> DRVTTQTAGNTAINTQSSLGVLCAYVEDPTKSDPPSSSTDQPTTTFTAIDRWYTGRLNSWTKAVKTFSFQAVPLPGAFLSRQGGLNGGAFTATLHRHFLMKCGWQVQVQCNLTQFHQGALLVAMVPETTLDVKPDGKAKSLQELNEEQWVEMSDDYRTGKNMPFQSLGTYYRPPNWTWGPNFINPYQVTVFPHQILNARTSTSVDINVPYIGETPTQSSETQN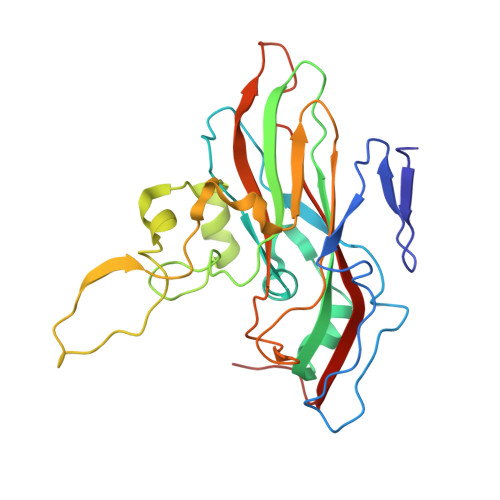SWTLLVMVLVPLDYKEGATTDPEITFSVRPTSPYFNGLRNRYTA> MGHHHHHHNNTEFYDRLGVSKNASADEIKKAYRKLSKKYHPDINKEPGAEDKYKEVQEAYETLSDDQKRAAYDQYGAAGANGGFGGAGGFGGFNGAGGFGGFEDIFSSFFGGGGSSRNPNAPRQGDDLQYRVNLTFEEAIFGTEKEVKYHREAGCRTCNGSGAKPGTSPVTCGRCHGAGVINVDTQTPLG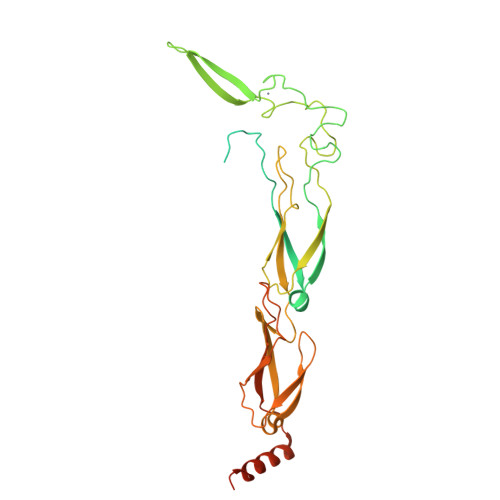MMRRQVTCDVCHGRGKEIKYPCTTCHGTGHEKQAHSVHVKIPAGVETGQQIRLAGQGEAGFNGGPYGDLYVVVSVEASDKFEREGTTIFYNLNLNFVQAALGDTVDIPTVHGDVELVIPEGTQTGKKFRLRSKGAPSLRGGAVGDQYVTVNVVTPTGLNDRQKVALKEFAAAGDLKVNPKKKGFFDHIKDAFDGE>MAKRSLRKMWRPGEKKEPQGVVYEDVPDDTEDFKESLKVVFEGSAYGLQNFNKQKKLKRCDDMDTFFLHYAAAEGQIELMEKITRDSSLEVLHEMDDYGNTPLHCAVEKNQIESVKFLLSRGANPNLRNFNMMAPLHIAVQGMNNEVMKVLLEHRTIDVNLEGENGNTAVIIACTTNNSEALQILLKKGAKPCKSNKWGCFPIHQAAFSGSKECMEIILRFGEEHGYSRQLHINFMNNGKATPLHLAVQNGDLEMIKMCLDNGAQIDPVEKGRCTAIHFAATQGATEIVKLMISSYSGSVDIVNTTDGCHETMLHRASLFDHHELADYLISVGADINKIDSEGRSPLILATASASWNIVNLLLSKGAQVDIKDNFGRNFLHLTVQQPYGLKNLRPEFMQMQQIKELVMDEDNDGCTPLHYACRQGGPGSVNNLLGFNVSIHSKSKDKKSPLHFAASYGRINTCQRLLQDISDTRLLNEGDLHGMTPLHLAAKNGHDKVVQLLLKKGALFLSDHNGWTALHHASMGGYTQTMKVILDTNLKCTDRLDEDGNTALHFAAREGHAKAVALLLSHNADIVLNKQQASFLHLALHNKRKEVVLTIIRSKRWDECLKIFSHNSPGNKSPITEMIEYLPECMKVLLDFCMLHSTEDKSCRDYYIEYNFKYLQCPLEFTKKTPTQDVIYEPLTALNAMVQNNRIELLNHPVCKEYLLMKWLAYGFRAHMMNLGSYCLGLIPMTILVVNIKPGMAFNSTGIINETSDHSEILDTTNSYLIKTCMILVFLSSIFGYCKEAGQIFQQKRNYFMDISNVLEWIIYTTGIIFVLPLFVEIPAHLQWQCGAIAVYFYWMNFLLYLQRFENCGIFIVMLEVILKTLLRSTVVFIFLLLAFGLSFYILLNLQDPFSSPLLSIIQTFSMMLGDINYRESFLEPYLRNELAHPVLSFAQLVSFTIFVPIVLMNLLIGLAVGDIAEVQKHASLKRIAMQVELHTSLEKKLPLWFLRKVDQKSTIV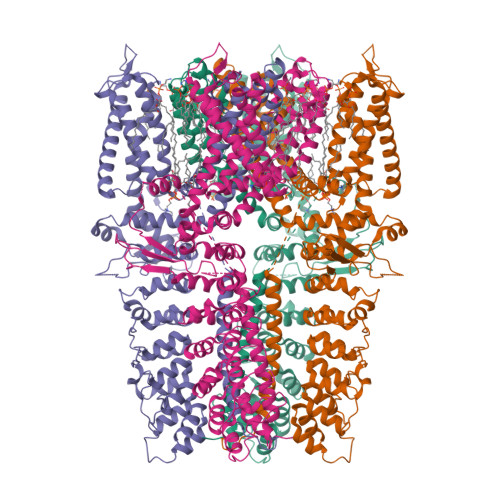YPNKPRSGGMLFHIFCFLFCTGEIRQEIPNADKSLEMEILKQKYRLKDLTFLLEKQHELIKLIIQKMEIISETEDDDSHCSFQDRFKKEQMEQRNSRWNTVLRAVKAKTHHLEPSNSLEVLFQGPAADYKDDDDKAHHHHHHHHHH[4x]>MPFITVGQENSTSIDLYYEDHGTGTPVVLIHGFPLSGHSWERQSAALLDAGYRVITYDRRGFGQSSQPTTGYDYDTFAADLNTVLETLDLQDAVLVGFSMGTGEVARYVSSYGTARIAAVAFLASLEPFLLKTDDNPDGAAPQEFFDGIVAAVKADRYAFYTGFFNDFYNLDENLGTRISEEAVRNSWNTAASGGFFAAAAAPTTWYTDFRADIPRIDVPALILHGTGDRTLPIENTARVFHKALPSAEYVEVEGAPHGLLWTHAEEVNTALLAFLAKAQEAQKQKLLTEVETYVLSIIPSGPLKAEIAQRLEDVFAGKNTDLEVLMEWLKTRPILSPLTKGILGFVFTLTVPSERGLQRRRFVQNALNGNGDPNNMDKAVKLYRKL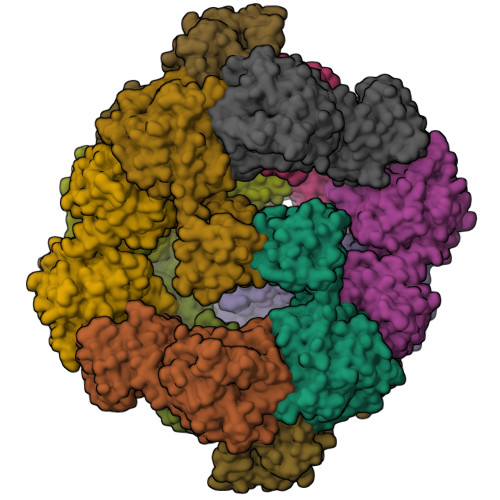KREITFHGAKEISLSYSAGALASCMGLIYNRMGAVTTEVAFGLVCATCEQIADSQHRSHRQLEHHHHHH[12x]> GHMKSDIPLFVQPEDFGTIQIEVLSTLYRDNEDDLSILIAIIDRKSGKEMFKFSKSIHKVRELDVYMKSHVPDLPLPTLPDRQLFQTLSPTKVDTRKNILNQYYTSIFSVPEFPKNVGLKIAQFISTDTVMTPPMMDDNVKDGSLLLRRPKTLTGNSTWRVRYGILRDDVLQLFDKNQLTETIKLRQSSIELIPNLPEDRFGTRNGFLITEHKKSGLSTSTKYYICTETSKERELWLSAFSDYIDPSQSLSLSSSRNANDT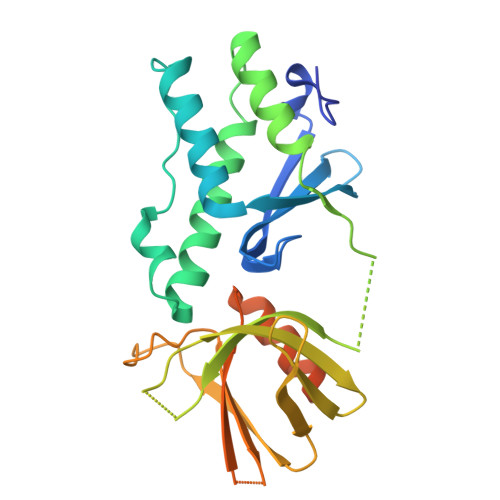DSASHLSA>GSATVTVTFTITELCLRTGVSEEELTEIVGLGMIEPHQPQADTWLFDDSAVTIVHRAVRLRNELELDWPGIAVALTLLDENARLTRENRLLQQRLARFLAHG[2x];>GSELKDYYAIMGVKPTDDLKTIKTAYRRLARKYHPDVSKEPDAEARFKEVAEAWEVLSDEQRRAEYDQMWQHRN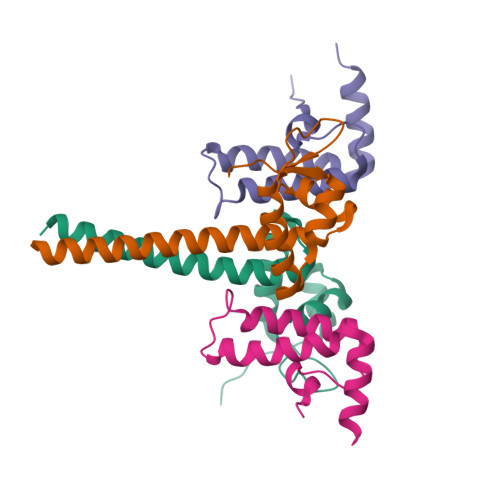[2x]The serine-rich repeat (SRR) glycoproteins of Gram-positive bacteria are an expanding family of microbial adhesins and virulence factors. Three of the SRR proteins (GspB of Streptococcus gordonii strain M99, Hsa of S. gordonii strain Challis, and SrpA of Streptococcus sanguinis strain SK36) bind human platelets through their interaction with glycocalicin, which is the carbohydrate-rich extracellular portion of the platelet membrane glycoprotein GPIbα. Among the best characterized of the SRR adhesins is GspB from S. gordonii, which has demonstrated binding affinity for the sialyl-T antigen carbohydrate decorating platelet glycoprotein GPIbα. Binding of these SRR adhesins to platelets is a high affinity process, with the interaction between GspB and glycocalicin having a KD of 2.38×10−8 M and appears to be a major factor in the pathogenesis of infective endocarditis, since the loss of GspB or Hsa expression results in a marked reduction in virulence.

Here, we report the high-resolution crystal structure of GspBBR, both alone and in complex with the disaccharide α-2,3-sialyl (1-thioethyl)galactose, a precursor to synthetically-produced sialyl-T antigen. Our analysis of the structure further identified that GspBBR contains an unusually modular fold, prompting us to re-analyze the sequences of the SRR family of adhesins. While still predominated by β-strands, the C-terminal subdomain of GspBBR does not contain an Ig-fold. A comparison of the structure of GspBBR determined with and without the disaccharide did not show significant structural changes localized within the binding pocket, which suggests that it is pre-formed. We determined that other structurally uncharacterized SRR adhesins also contain modules within their binding regions, suggesting that particular subdomains may be included, removed, or interchanged, manifesting in the broad range of binding partners observed in the family. Importantly, the structure of GspBBR provides insight into the binding repertoire of other SRR proteins, and specifically highlights which modules mediate binding to host carbohydrate receptors.

> RAVTESAPNVEYHDVKGDMIQSVTTSFDDTSRLLTWTINLTPRQVKSNLGALVSISGNQETRTVTINGKNAANGGVYNSGGAWNLYTGESVNNNVLRITTQVNDTGGEVKLGLRLVTSDKKITKTNLPLEFSQVAATTNGSWDKAGYNTTIVEKDTERPVVNVPSEITVYRGESFEYFATVTDNSNAFDLAKTVVRWLYSNQPGRGTEWLQYSVTQVGNQLKVRIFGNVPIDTTIGDYTRYVVATDAAGNVNATQTEMGNAAVDKTSVNGQFKLIIRFRIKTPENTVFVNNPNQLTEVEKNLVREAVKKSNPDLRAQDVLNSNYVTGITVSNNGTTTITYRDGRKDIIDGSKFIDTRAGS>[2x]MHHHHHHIPRNLLNAYAGPNALRDYFDPDCQPMIPLVEIPQSLNPFYEDGVRIHAKMMSMHPSNNVKIMPALNMLTKEVQPEKSKTVIEYSSGSTVISLALVSRINHGINDVRAFLSNKT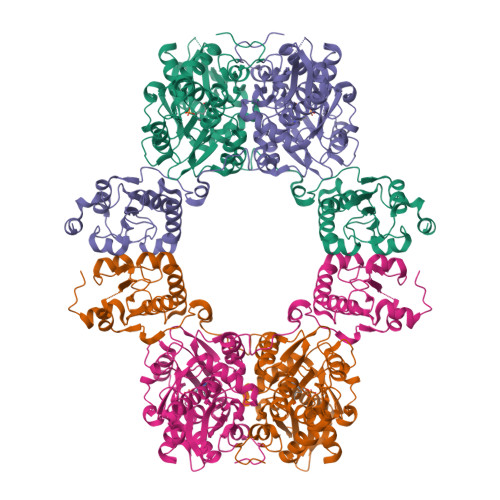SAPKLRLMQFFGLDVTLFGGPSQPAPNDERGGIYRARMMAREDEAILNVDQYENDANWQSHVKWTGPQIHEQLPSIRLICAGMGTSGTMTGLGQYFKTAKPSVFRLGVCTAAGDRVPGPRSLALLSPVEFPWRDSVDAIEEVGSKDAFTLSLKLCREGLICGPSSGFNLQGLFNYLGRLKAAGTLSSLAGPYGIIDCAFICCDLPYPYVDEYFDKLGDNAFHPIRNQNLAAVDLYRYDEAWELEPSSALSHFTSSTHGVEAVLLDLRKPEDFIMSHIPGSYNLPLQSSNASTPSPFTDAMVLEKQWKELEATFTLDRINAHDLSGKDVYILCYNGDTARVATSVLRAKGISASSVKGGIAAVRKDLPQMQMAERGRVLVQQDWIKTPEIVAKELRVDSLSPAARGPNEITV>[2x]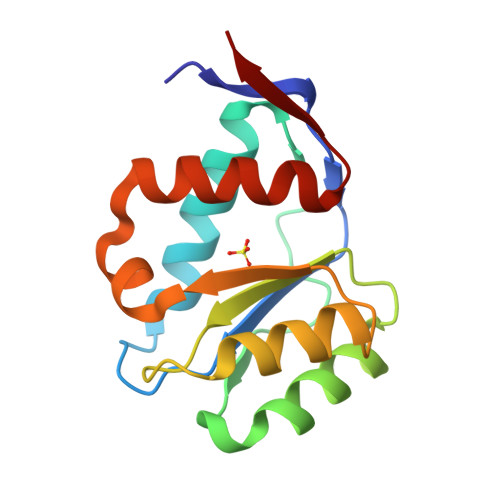SDKKMVNGAKVTSWTCVSFSTRIDRGLPQEFCKQLIGMCVSKGMEFKPQPAIPFISCPPEHIEEALLDIHKRAPGLQLLIVILPDVTGSYGKIKRICETELGIVSQCCQPRQVNKLNKQYMENVALKINVKTGGRNTVL>VTAYEEIVCQVFAAVLDRSDVTADADFFALGGHSLLSLRVVARLRALLGVDVGVRDLFEAPTPAALAARLTTQTGRRPAVTRRGPDAPPVLSHFQRGLWLIEQVYQTRGAYNVPLAVHVSDRLDLDVLRAAVRDLVARHEVLRTLVRSSDDGPDPVLLAPEDAAVDVAEVQAAGPVADLLAELTAQPFDLATQIPLRVRMITGEQVDGCVLLLVCHHIAADEWSFAPLLRDLDTAYRARAAGRAPDWEPLPAQYSDYAATLHDWLGEATDPASPLRRQLDYWQHALQDLPDELDLPTDRPRPATASHRGGLARAELPPELVEAVRRLAAQHGVTVFMVVQAAVAVLLHRLGAGDDIPLGSPVADRADEAVHDTVGFFL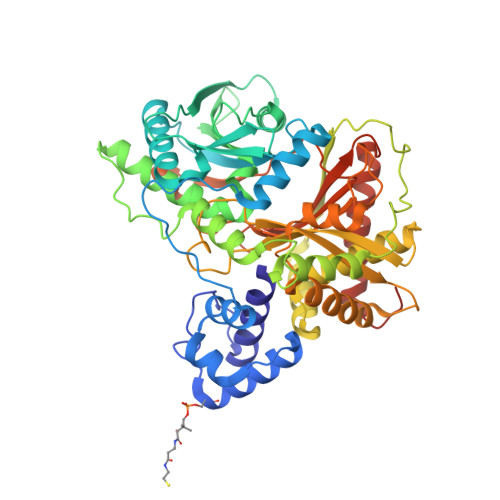NTLVLRVNLSGNPTFADLLDRVRAVDLEAFARADAPFDAVVDTVKPPRAVSRHPLFQTMVSYQRRPSDVDRLFGAATRLVEVPLDTAKFDLEFAFIEDGHGGAHIALNYAADLFDHDSAEQLVARLRTVLEHACADPCRPVAGVEVVSGA[2x]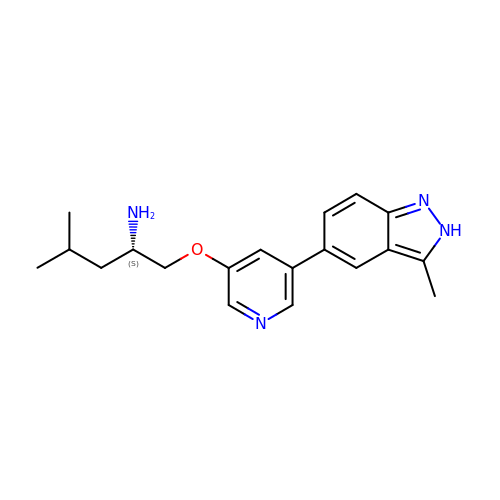(2~{S})-4-methyl-1-[5-(3-methyl-2~{H}-indazol-5-yl)pyridin-3-yl]oxy-pentan-2-amine | C19 H24 N4 O | CEDLXWRFEZCVEU-INIZCTEOSA-N> RVADTVGTGPTNSEAIPALTAAETGHTSQVVPGDTMQTRHVKNYHSRSESTIENFLC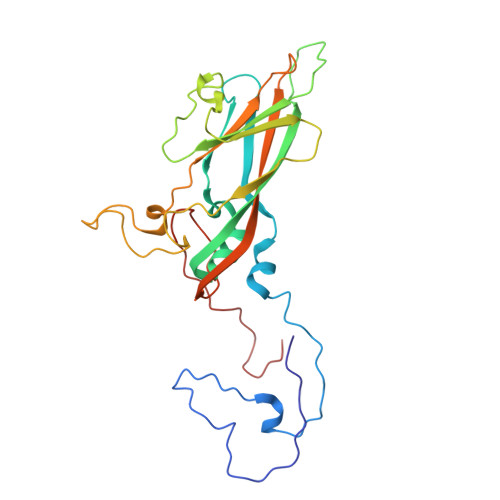RSACVYFTEYENSGAKRYAEWVLTPRQAAQLRRKLEFFTYVRFDLELTFVITSTQQPSTTQNQDAQILTHQIMYVPPGGPVPDKVDSYVWQTSTNPSVFWTEGNAPPRMSIPFLSIGNAYSNFYDGWSEFSRNGVYGINTLNNMGTLYARHVNAGSTGPIKSTIRIYFKPKHVKAWIPRPPRLCQYEKAKNVNFQPSGVTTTRQSITTMT> MTSALLVASRRARQAQGLPRCLLHAIGIHAGTRAEFASVALQEAGTTPSTSGQEQPSSAQLTPAHLRSYYPLNLALLPEAARGSAGAFYTPRDPGHERRGGCKALQQEMEATGRASILYRPIMAALNGAVAAGQQPRLLLTGPAGCGKSLALLGLVEWARQQGWLVVYVPSCLALVRGGYFARRGRGAAGGWDT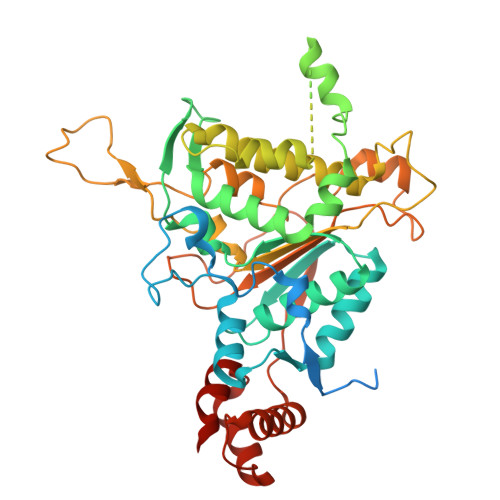LTSAQQLLKGVMDAHGPLLQSLPVLPVPGRAARRQQQQQHEPRQADKPAKVEEGQGQGQGQAGGSGLLEEGSGSASGAGGGGGRTLQDVALRGLSSDDNAQLAVDSALQLIRQLQLLGSGAAQPPDSQPGQPPRVLFALDDYNYLYGPTDYGVQPPSASPLQGRRRVLDAGELILARGLRLLESELGTNPVAAAAAGGGAGGVGGAVVVAATTATPALPAPRSLALEVPHTVVEVPGFDEAETAAALAHYAATGAATRAASAAEARHLFALTGGNGRELRAKAGALGVRVG>[6x]SVKHQQAVDETLTPWTWNNNNFSSLKITGENPGSFGLVRSQNDNLNISSVTKNSSDDNLKYLNAVEKYLDGQQNFAIRRYDNNGRALYDINLAKMENPSTVQRGLNGEPIFDPFKGFGLTGNAPTDWNEIKGKVPVEVVQSPHSPNLYFVLLVPKVALEYHNLNNQVVKESLE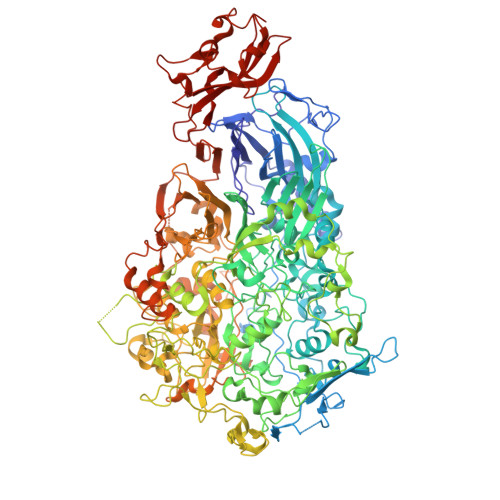VKATQSSFNPTQRLQKDSPVKDSSKQGEKLSETTASSMSSGMATSTRAKALKVEVERGSQSDSLLKNDFAKKPLKHKNSSGEVKLEAEKEFTEAWKPLLTTDQIAREKGMGATVVSFYDAPYSENHTAFGLVDHIDPKKMVENYPPSWKTPKWNHHGIWDYNARNLLLQTTGFFNPRRHPEWFDEGQAKADNTSPGFKVGDTDHKKDGFKKNSSSPIALPFEAYFANIGNMVAIGNSVFIFGGNGHATKMFTTNPLSIGVFRIKYTDNFSKSSVTGWPYAVLFGGLINPQTNGLKDLPLGTNRWFEYVPRMAVSGVKWVGNQLVLAGTLTMGDTATVPRLKYDQLEKHLNLVAQGQGLLREDLQIFTPYGWANRPDIPVGAWLQDEMGSKFGPHYFLNNPDIQDNVNNDTVEALISSYKNTDKLKHVYPYRYSGLYAWQLFNWSNKLTNTPLSANFVNENSYAPNSLFAAILNEDLLTGLSDKIFYGKENEFAENEADRFNQLLSLNPNPNTNWARYLNVVQRFTTGPNLDSSTFDQFLDFLPWIGNGKPFSNSPSPSTSASSSTPLPTFSNINVGVKSMITQHLNKENTRWVFIPNFSPDIWTGAGYRVQSANQKNGIPFEQVKPSNNSTPFDPNSDDNKVTPSGGSSKPTTYPALPNSISPTSDWINALTFTNKNNPQRNQLLLRSLLGTIPVLINKSGDSNDQFNKDSEQKWDKTETNEGNLPGFGEVNGLYNAALLHTYGFFGTNTNSTDPKIGFKADSSSSSSSTLVGSGLNWTSQDVGNLVVINDTSFGFQLGGWFITFTDFIRPRTGYLGITLSSLQDQTIIWADQPWTSFKGSYLDSDGTPKSLWDPTALKSLPNSSTTYDTNPTLSPSFQLYQPNKVKAYQTTNTYNKLIEPVDATSAATNMTSLLKLLTTKNIKAKLGKGTASSQGNNNGGGVSQTINTITTTGNISEGLKEETSIQAETLKKFFDSKQNNKSEIGIGDSTFTKMDGKLTGVVSTPLVNLINGQGATSDSDTEKISFKPGNQIDFNRLFTLPVTELFDPNTMFVYDQYVPLLVNLPSGFDQASIRLKVISYSVENQTLGVRLEFKDPQTQQFIPVLNASSTGPQTVFQPFNQWADHHHHHH> RIIGGSDADIKNFPWQVFFDNPWAGGALINEYWVLTAAHVVEGNREPTMYVGSTSVQTSRLAKSKMLTPEHVFIHPGWKLLEVPEGRTNFDNDIALVRLKDPVKMGPTVSPICLPGTSSDYNLMDGD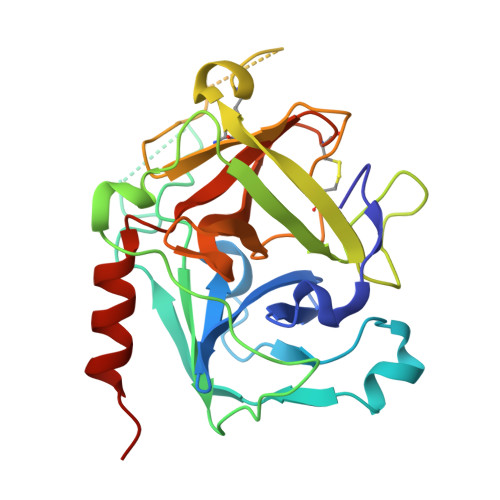LGLISGWGRTEKRDRAVRLKAARLPVAPLRKCKEVKVEKPTADAEAYVFTPNMICAGGEKGMDSCKGDSGGAFAVQDPNDKTKFYAAGLVSWGPQCGTYGLYTRVKNYVDWIMKTMQENSTPRED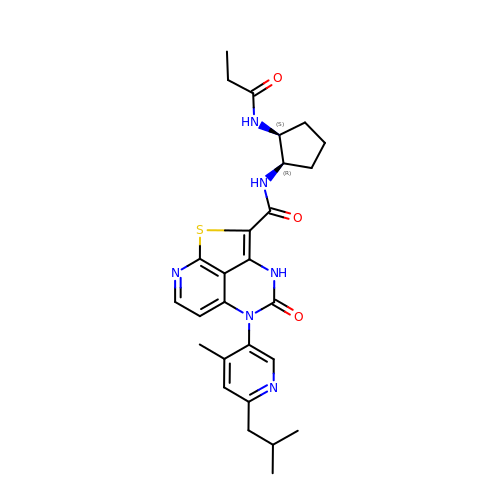(5P)-5-[4-methyl-6-(2-methylpropyl)pyridin-3-yl]-4-oxo-N-[(1R,2S)-2-propanamidocyclopentyl]-4,5-dihydro-3H-1-thia-3,5,8-triazaacenaphthylene-2-carboxamide | C27 H32 N6 O3 S | KBWVWXCEDLZVBM-ZWKOTPCHSA-N> HPYYLRSFLVVLKTVLENEDDMLLFDEQEKGIVTKFYQLSATGQKLYVRLFQRKLSWIKMTKLEYEEIALDLTPVIEELTNAGFLQTESELQELSEVLELLSAPELKSLAKTFHLVNPNGQKQQLVDAFLKLAKQHSVCTWGKNKPGIGAVILKRAKALAGQSVRICKGPRAVFSRILLLFSLTDSMEDEDAACGGQGQLSTVLLVNLGRMEFPSYTINRKTHIFQDRDDLIRYAAATHMLSDISSAMANGNWEEAKELAQCAKRDWN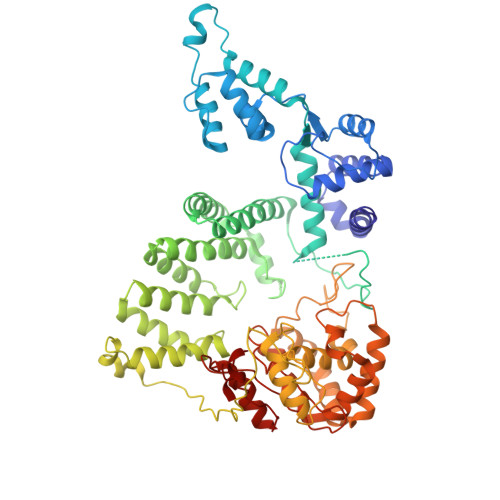RLKNHPSLRCHEDLPLFLRCFTVGWIYTRILSRFVEILQRLHMYEEAVRELESLLSQRIYCPDSRGRWWDRLALNLHQHLKRLEPTIKCITEGLADPEVRTGHRLSLYQRAVRLRESPSCKKFKHLFQQLPEMAVQDVKHVTITGRLCPQRGMCKSVFVMEAGEAADPTTVLCSVEELALAHYRRSGFDQGIHGEGSTFSTLYGLLLWDIIFMDGIPDVFRNACQAFPLDLCTDSFFTSRRPALEARLQLIHDAPEESLRAWVAATWHEQEGRVASLVSWDRFTSLQQAQDLVSCLGGPVLSGVCRHLAADFRHCRGGLPDLVVWNSQSRHFKLVEVKGPNDRLSHKQMIWLAELQKLGAEVEVCHVVAVGAKSQSLS> MTEKEEKEDLQAQDKEEQQIKADTKVISVQEFEEYMRFKEQANSKSKETSRDLSINERITKELAEVEERERIEKQLLLEAERINEIDTLAKAHLSNHFNKEVLLAKGYTLKDIMQAQRRELVRKFVPIEQIKAIAKVSDISHIDGEILEQLVSLAKVNIKLRKNASSSSSSVDSIKGNIAIKSEERASLLDSNFVPINFTE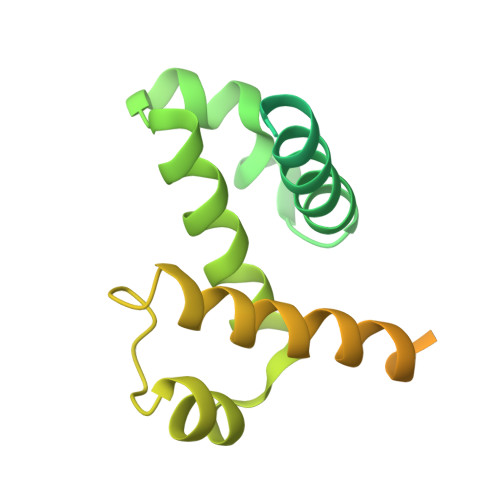FVQAISNTYKQRRIQFYENLKRHKRTSIA> AQQFQTIALIGIGLIGSSIARDIREKQLAGTIVVTTRSEATLKRAGELGLGDRYTLS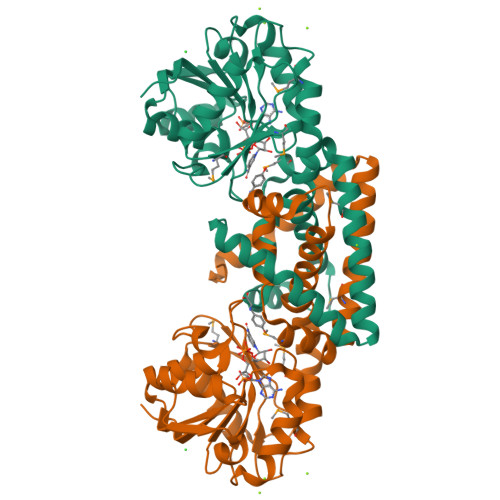AAEAVEGADLVVVSVPVGASGAVAAEIAAHLKPGAIVTDVGSTKGSVIAQMAPHLPKDVHFVPGHPIAGTEHSGPDAGFAGLFRGRWCILTPPAGTDEEAVARLRLFWETLGSMVDEMDPKHHDKVLAIVSHLPHIIAYNIVGTADDLETVTESEVIKYSASGFRDFTRLAASDPTMWRDVCLHNKDAILEMLARFSEDLASLQRAIRWGDGDKLFDLFTRTRAIRRSIVQAGQDT> GGVDMPERFDAFICYCPSDIQFVQEMIRQLEQTNYRLKLCVSDRDVLPGTCVWSIASELIEKRCRRMVVVVSDDYLQSKECDFQTKFALSLSPGAHQKRLIPIKYKAMKKEFPSILRF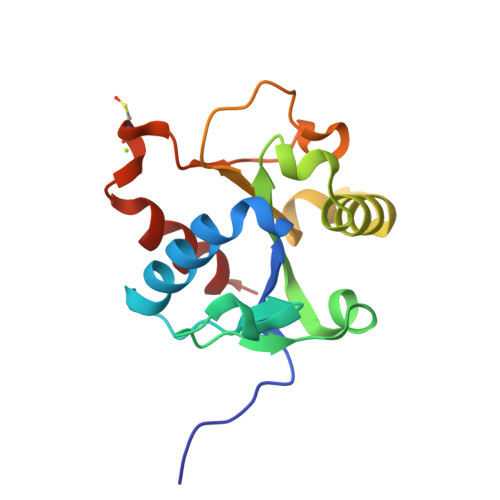ITVCDYTNPCTKSWFWTRLAKALSLP(2~{R},3~{S},4~{R},5~{R},6~{S})-2-(hydroxymethyl)-6-[5-(4-methoxyphenyl)-1~{H}-1,2,4-triazol-3-yl]oxane-3,4,5-triol | C15 H19 N3 O6 | 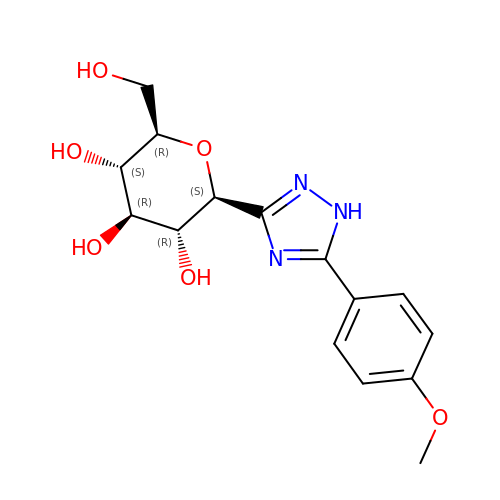YPWXLHANNFWVLG-UJPOAAIJSA-N The Notch signalling pathway is highly conserved and plays key roles in many aspects of development and homeostasis. Canonical Notch signalling involves a simple cascade, whereby ligand binding induces successive cleavages to release the Notch intracellular domain (NICD) which translocates to the nucleus and directly regulates gene expression with its binding partners (Kovall, 2008; Kovall & Blacklow, 2010; Bray, 2016; Kovall et al, 2017). All Notch ligands have a similar architecture, with an extracellular domain consisting of multiple (7, 8, or 16) epidermal growth factor (EGF) repeats, a so‐called Delta/Serrate/Lag‐2 (DSL) domain and a highly conserved N‐terminal region (Bray, 2006; D’Souza et al, 2008; Kopan & Ilagan, 2009; Kovall & Blacklow, 2010). Receptor binding involves the N‐terminal portion including the DSL and N‐terminal domains (Cordle et al, 2008; Luca et al, 2015, 2017).

To determine whether the Drosophila ligands adopt the same arrangement as their mammalian counterparts, we solved the structures of the N‐terminal region of Drosophila Delta and Serrate as well as the ligand‐binding region of Drosophila Notch (EGF11‐13; Fig EV1A–E). These were solved using molecular replacement of the individual domains from the human homologues to resolutions between 1.5 and 3.0 Å. The conserved domain arrangement allows us to model the Notch–ligand complex by overlay of the Drosophila structures on the earlier structures of the mammalian complexes (Luca et al, 2015, 2017) with this leading to no significant clashes between the Notch and ligand coordinates. In B, C, E, Glycosylation is shown in a stick representation as are the side chains to which the glycans are attached and disulphide bonds. Purified Delta (NE3 fragment) also exhibited robust binding to a fragment of Drosophila Notch (dNotch EGF11‐13), which contains the core ligand‐binding sites. This relies on the conventional contact sites because it is abolished by an alanine substitution in the DSL domain which replaces a key receptor‐binding residue (F204).

> DIDECDQGSPCEHNGICVNTPGSYRCNCSQGFTGPRCETNINECESHPCQNEGSCLDDPGTFRCVCMPGFTGTQCEIDIDECQSNPCLNDGTCHDKINGFKCSCALGFTGARCQIN>[4x]MRYADRVAGISWETIEEVRRRLKERPALHFIAGEFVPSESGETFPSLDPATNEVLGVAARGGEREVDRAAKAAHEAFQRWSRTKAKERKRYLLRIAELIEKHADELAVMECLDAGQVLRIVRAQVARAAENFAFYAEYAEHAMEDRTFPVDRDWLYYTVRVPAGPVGIITPWNAPLMLSTWRIAPALAFGNTVVLKPAEWSPFTATKLAEILKEADLPPGVFNLVQGFGEEAGAALVAHPLVPLLTLTGETETGKIVMRNAADHLKRLSPELGGKSPALVFADADLERALDAVVFQIFSFNGERCTASSRLLVEEKIFEDFVGKVVERARAIRVGHPLDPETEVGPLIHPEHLQRVLGYVEAGKREGARLLVGGERAKTSFRGEDLSRGNYLLPTVFVGENHMKIAQEEIFGPVLVAIPFKDEEEALRKANDTKYGLAAYVFTRDLERAHRLALELEAGMVYLNSHNVRHLPTPFGGVK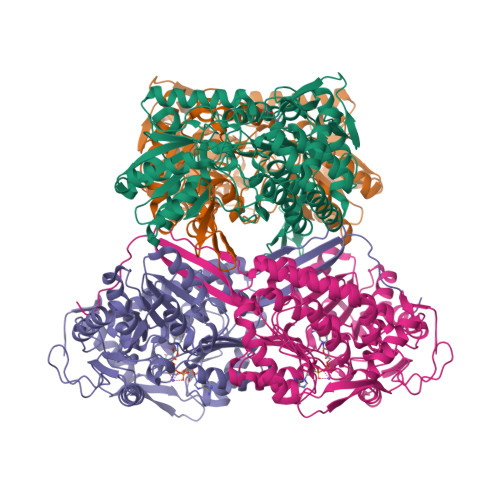GSGDRREGGTYALDFYTDLKTIALPLRPPHVPKFGK> SDRVRSITLGNSTITTQECANVVVGYGVWPDYLSDEEATAEDQPTQPDVATCRFYTLNSVKWEMQSAGWWWKFPDALSEMGLFGQNMQYHYLGRSGYTIHVQCNASKFHQ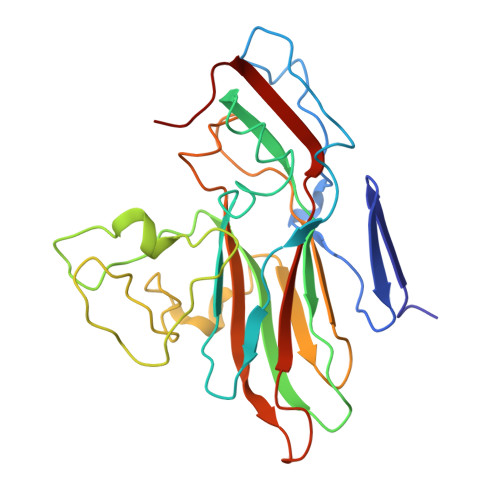GCLLVVCVPEAEMGCTNAENAPTYGDLCGGETAKQFEQNAVTGETAVQTAVCNAGMGVGVGNLTIYPHQWINLRTNNSATIVMPYINSVPMDNMFRHNNFTLMIIPFAPLDYVTGASSYIPITVTVAPMSAEYNGLRLAGHQ> MSTISREEYAKKMRLALSDNHICKPDGTVNHQYFLVKKGQYWGEEKIQYLIEQLEKIGVGNWKQMQKGLLEQTSEIEL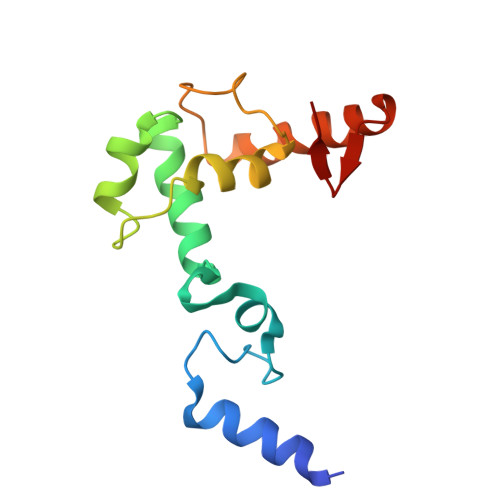ELRTCLLFKTTDIQPYMDKKFTKIEIEQIAQQNIEKAQQLSKLKYGVFVV>[2x]GTSSMADIGSELGFNEAERQKILDSNSSLMGNANEVRDKFIQNYASSLKDSNDPQDFLRRVQELRINMQKNFISFDVYYNYLNNLVLASYNRCKQEKTFAESTIKNE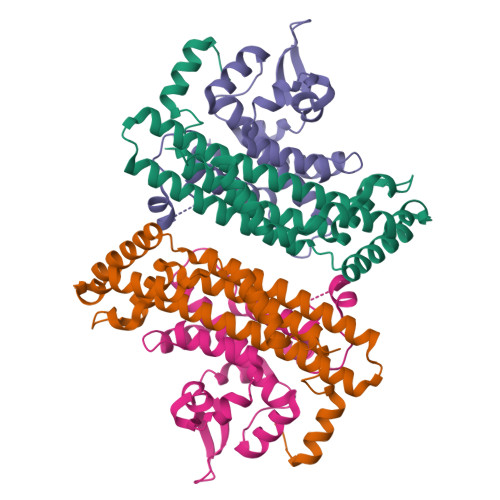LTLGEFVAEISDNFNNFMCDEVARISDLVASYLPREYLPPFIDGNMMGVAFQILGIDDFGRKLNEIVQDIGTKYIILSKNKTYLTSLERAKLITQLKLNLE;>[2x]GTSSMADIGSEPFSLKTHRFNPFAYVDFGNDVVLTEDILSQIDTRLKGHGMVASGGDFSTQIFGLAKLVFPERPNEKDPFFSNQARNLFVINCNIYRDLMWTKKGLEFVKRKKIIMPETPTMFFIGSMASGINLIDEDTNMEKVVSLMEFFGGEEDKSGDNLRVLSPATRNMWNSFKTMGGARETYSSVQGVYTSAFAPYNNAMIRNFTS> MGSHHHHHHGRSMVAGHASGSPAFGTASHSNSEHEEIHLAGSIQPHGALLVVSEHDHRVIQASANAAEFLNLGSVLGVPLAEIDGDLLIKILPHLDPTAEGMPVAVRCRIGNPSTEYCGLMHRPPEGGLIIELERAGPSIDLSGTLAPALERIRTAGSLRALCDDTVLLFQQCTGYDRVMVYRFDEQGHGLVFSECHVPGLESYFGNRYPSSTVPQMARQLYVRQRVRVLVD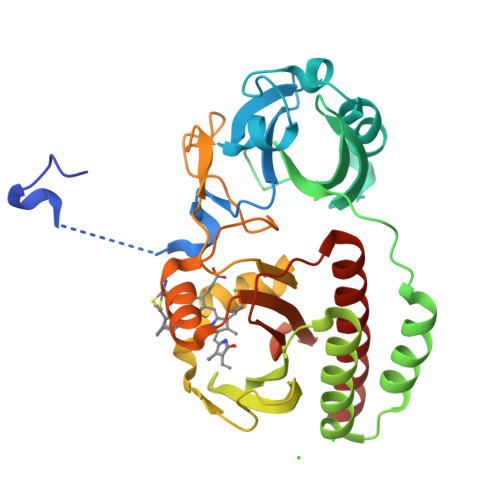VTYQPVPLEPRLSPLTGRDLDMSGCFLRSMSPCHLQYLKDMGVRATLAVSLVVGGKLWGLVVCHHYLPRFIRFELRAICKRLAERIATRITALES S-DIOXYMETHIONINE | C5 H11 N O4 S | 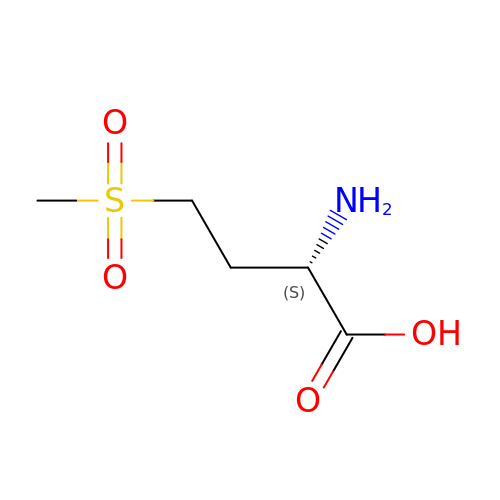UCUNFLYVYCGDHP-BYPYZUCNSA-N>[4x]DITDKNQSIDSGISSLSYNRNEVLASNGDKIESFVPKEGKKAGNKFIVVERQKRSLTTSPVDISIIDSVNDRTYPGALQLADKALVENRPTILMVKRKPININIDLPGLKGE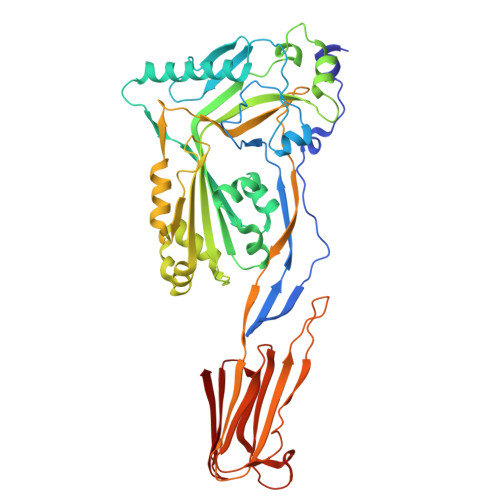NSIKVDDPTYGKVSGAIDELVSKWNEKYSSTHTLPARTQYSESMVYSKSQISSALNVNAKVLENSLGVDFNAVANNEKKVMILAYKQIFYTVSADLPKNPSDLFDDSVTFNDLKQKGVSNEAPPLMVSNVAYGRTIYVKLETTSSSKDVQAAFKALIKNTDIKNSQQYKDIYENSSFTAVVLGGDAQEHNKVVTKDFDEIRKVIKDNATFSTKNPAYPISYTSVFLKDNSVAAVHNKTDYIETTSTEYSKGKINLDHSGAYVAQFEVAWDEVSYDKEGNEVLTHKTWDGNYQDKTAHYSTVIPLEANARNIRIKARECTGLAWEWWRDVISEYDVPLTNNINVSIWGTTLYPGSSITYN N-[(4-{[(2-amino-4-oxo-3,4-dihydro[1]benzothieno[2,3-d]pyrimidin-5-yl)methyl]amino}phenyl)carbonyl]-L-glutamic acid | C23 H21 N5 O6 S | 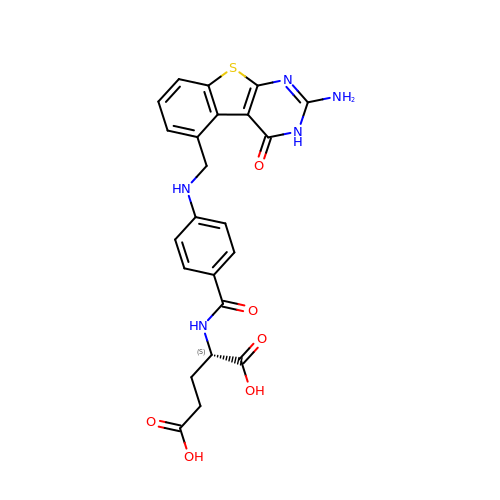GLRZVZIDWYADTN-AWEZNQCLSA-N> GMEFNHLTKQLNQLLAQDYVAFSITENPVVQMLSQASFA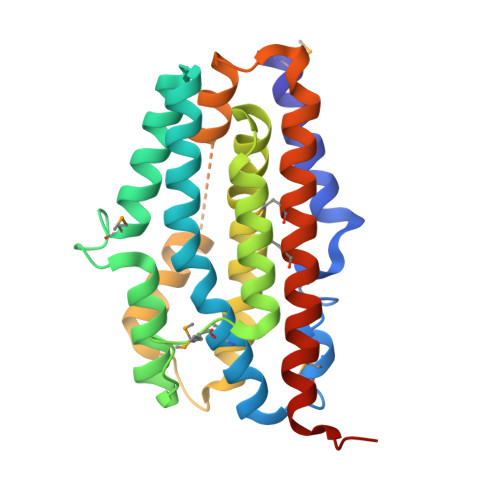QIAYVMQQYSIFPKELVGFTELARRKALGAGWNGVAQELQENIDEEMGSTTGGISHYTLLADGLEEGLGVAVKNTMPSVATSKLLRTVLSLFDRQVDYVLGATYAIEATSIPELTLIVKLVEWLHEGAIPKDLQYFFSKHLDEWEIEHEAGLRTSVAAYIQPEEFGEFAAGFRAMIDAMQVWWQELAQEAISSEVVLSTAIAQHH>HMAQDMRSEKRGLAYGYHSENDLKAMQGKVKWWYNWDTQADANVKENYASYGYDFVPMAWDENFNEEALRSFLDNHPDVKYLLGWNQPNFMEQANLTPAEAAAHWPVLEAIAQDYNLKLVAPAVNYSPGNVDIPGTDDDYDPWLYLDAFFEACEGCQVDYIAVHCYMKYESAFSWYVGEFERYNKPIWVTEWAGWDDGGPANMGEQMNFLSDTVRWMESNDNIYRYSWFLGRSSEGYDQFPYLDVLLADGELTPLGSVYTSIPSNDFRYKIPARIEAEGAHSLTGFKHLATTDTTGLAKLIAASNEVAEYKLNVEEGGDYTLALRLASSANSDIAIRVDGLLVYTFEDINTGGVEAWMTFSSTPISLTAGDHILRVESKSSRFGFNWLELTN[2x]

Our previous work revealed a curdlan-specific endo-β-1,3-glucanase, CBM6E, from a marine bacterium Saccharophagus degradans 2-40T, which contains an N-terminal GH128 module and a C-terminal CBM6 module. CBM6E exhibits catalytic activity at intermediate temperatures and efficiently produces GOS with DPs of 3–6 from curdlan. The CBM6 module of CBM6E (CBM6E-CBM6) exhibits a strong binding affinity specifically to curdlan, effectively enhancing the enzyme’s activity against curdlan. The GH128 and CBM6 modules form a cohesive structural entity, jointly recognizing triple-helical β-1,3-glucans.

The crystal structure of CBM6E complexed with GOS was obtained through cocrystallization of the E168Q inactive mutant of CBM6E with laminarihexaose (L6) and determined at a high resolution of 1.28 Å. This complex structure enabled the mapping of two β-1,3-GOS chains within the catalytic groove of the GH128 domain: one spanning from the -4 to -1 subsites and the other extending from the + 1 to + 5 subsites. The cleavage of the glycosidic bond between the − 1 and + 1 subsites might be attributed to residual enzyme activity of the E168Q mutant enzyme at high crystallization concentrations. The elongated catalytic groove of CBM6E aptly accommodates the curved conformations of the two GOS chains, which collectively form a single-helical structure. This structural characteristic correlates with CBM6E's preference for linear curdlan over branched laminarin, as well as its distinctive cleavage pattern yielding products L3 to L6. The interactions within the negative-subsite region are primarily governed by two conserved hydrophobic residues: W141, spanning from − 4 to − 2, and W117 at the − 2 subsite. The glucoside at the − 1 subsite establishes hydrogen bonds with N167, Q168, H245, and E272. Furthermore, a β-configuration is trapped within the − 1 subsite, which aligns with the retaining mechanism observed in the GH128 family. We were fortunate to observe glucosyl moieties from + 1 to + 5 in the complex structure of CBM6E. Furthermore, W256 and Y250 (corresponding to S198 and Y194 of PvGH128_II, respectively) provide aromatic platforms for the + 4 and + 5 glucosides, respectively.Despite these low concentrations, proteins have a great technological relevance in winemaking as some of them, the grape pathogenesis-related (PR) proteins, can aggregate to form a visible haze. Among the grape PR-proteins, the thaumatin-like proteins (TLPs) and chitinases can undergo changes in structural integrity, particularly under certain conditions such as when wines are exposed to elevated temperatures during storage or transportation. In this paper the crystal structure and some physico-chemical parameters relevant for the haze formation mechanism of three isoforms of TLPs isolated from grape juice were determined. Plant TLPs generally have three domains and a cleft located between domains I and II.

Despite sharing the same sequence, the two VVTL1 isoforms, I and H2 exhibited differences in their chromatographic behavior, a feature that allowed their separation and that also indicated that they possess some differences in physical properties. The physical differences between these two isoforms of the protein were also observed during crystallography. The initial solution for this structure was deposited in the Protein Data Bank as 4H8T. This initial structure included data to 2.0∶Å and an overall R value of 0.224. Domain I is the largest and forms the central core of the molecule. This domain comprises 11 β-strands forming a β-sandwich of two β-sheets. The two β-sheets are stabilized by four disulfide bonds (residues 33–224, 89–95, 140–213, and 146–196). Domain II consists of a long α-helix (α5) and four α-helical segments (α1 to α4), and is stabilized by four disulfide bonds (residues 146–196, 154–164, 168–177, 178–183). Importantly, disulfide bond 89–95 connects domain I to III, while disulfide bond 146–196 connects domain I to II. The comparison of the two structures performed with the algorithm for protein structure alignment and comparison named TM-align tool indicated that the two proteins have a root mean square deviation (RMSD) of 0.78 Å, with a TM-score of 0.98, indicating that the proteins belong to the same fold (thaumatin), confirming results previously obtained with CATH.

>ATFDILNKCTYTVWAAASPGGGRRLDSGQSWTITVNPGTTNARIWGRTSCTFDANGRGKCETGDCNGLLECQGYGSPPNTLAEFALNQPNNLDYIDISLVDGFNIPMDFSGCRGIQCSVDINGQCPSELKAPGGCNNPCTVFKTNEYCCTDGPGSCGPTTYSKFFKDRCPDAYSYPQDDKTSLFTCPSGTNYKVTFCP[2x]> MSPYSSDTTPCCFAYIARPLPRAHIKEYFYTSGKCSNPAVVFVTRKNRQVCANPEKKWV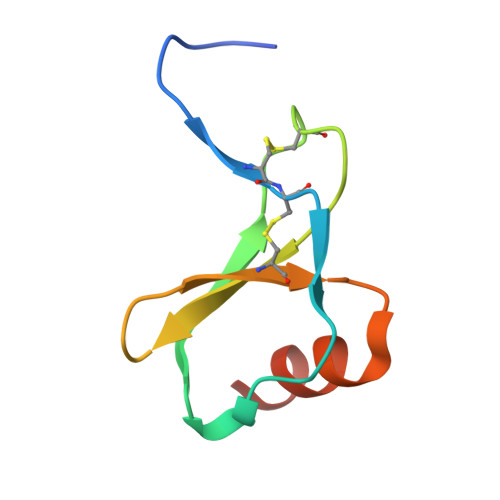REYINSLEMS> MEKDGLCRADQQYECVAEIGEGAYGKVFKARDLKNGGRFVALKRVRVQTGEEGMPLSTIREVAVLRHLETFEHPNVVRLFDVCTVSRTDRETKLTLVFEHVDQDLTTYLDKVPEPGVPTETIKDMMFQLLRGLDFLHSHRVVHRDLKPQNILVTSSGQIKLADFGLARIYSFQMALTSVVVTLWYRAPEVLLQSSY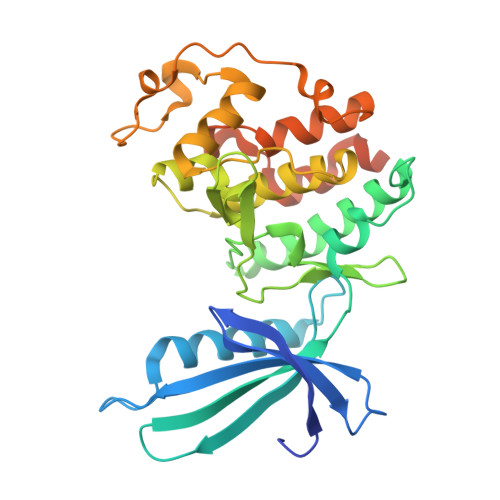ATPVDLWSVGCIFAEMFRRKPLFRGSSDVDQLGKILDVIGLPGEEDWPRDVALPRQAFHSKSAQPIEKFVTDIDELGKDLLLKCLTFNPAKRISAYSALSHPYFQDLERCKENLDSHLPPSQNTSELNTA[(1~{R})-3-(3,4-dimethoxyphenyl)-1-[3-(2-morpholin-4-ylethoxy)phenyl]propyl] (2~{S})-1-[[(1~{R},4~{a}~{R},8~{a}~{R})-4-oxidanylidene-2,3,4~{a},5,6,7,8,8~{a}-octahydro-1~{H}-naphthalen-1-yl]carbonyl]piperidine-2-carboxylate | C40 H54 N2 O8 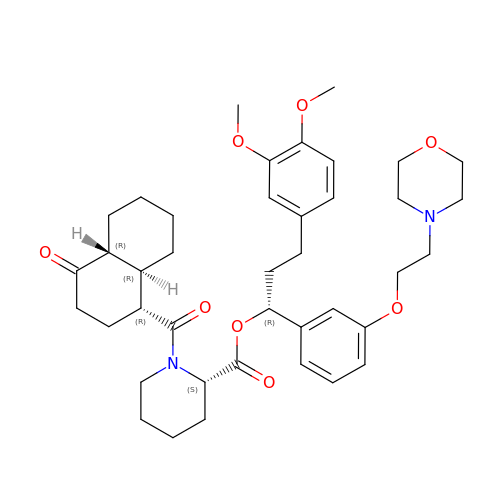| UGIVXHVIZXJHDG-YGYPXORBSA-N>NLYFQGAGAGAGAGAMSELSAIETAAAIAGGSMTALEACDAAIARIEQRDGPINAVVVRDFDRARDAAKAADAEIAAAVRKPLLGVPMTIKESFDIAGLPTSWGFAEHADHIATADSLVVSRLKAAGAVFLGKSNIPVGLADWQSVNPNYGRTNNPHDHSRSAGGSSGGAAAALAAGMVPLEYGSDIGGAIRVPAHFCGVWGLKTTFDAVSLEGHYFPRTDSAKADLSVVGPMARTPADLALALDITSKVPLPQSRIANLSGLRILLLTAHPETVADSATISAVERAAAACEASGATVATSSPDLPDLSALVADYTRMLLVVLARGLAPEGT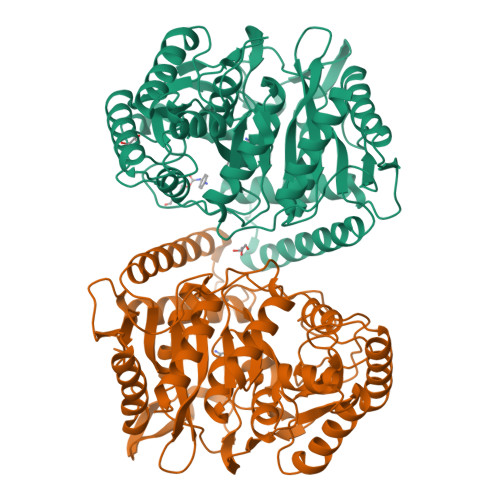EPVSLNAWYAMLDDQARMMRAFDRLFESFDAIFCPVLGTTAFAHSDEPDWAKRSLSIDGGIAPFAAQLGWISMATYGGMPALSMPLGADGNGLPINLQIITRNWSDHDAIRIGALVAEALDR[2x]> MDYKDDDDKDYKDDDDKDYKDDDDKLEVLFQGPGMSFKATITESGKQNIWFRAIYVLSTIQDDIKITVTTNELIAWSMNETDTTLCQVRFQKSFFEEYEFKPHEIVFGENGVQVIEDTYGNSHKLYSFRVNGRHLTTISRKPDGDGIKSFTIAVNNTSTCPESLANRLIVVIEMDSLIVKEYCPQFQPIKYDPIIINLKYKRRFLDVFGTAASDRNPQEPLDPKLLDVFTNTERELTSALFNEEVESDIRKRNQLTAADEINYICCNSTLLKNFLDNCNVNVTDEVKLEINVHRLSITAFTKAVYGKNNDLLRNALSMSNTISTLDLEHYCLFTTIEDEKQDKRSHSKRREHMKSIIFKLKDFKNFITIGPSWKTTQDGNDNISLWFCHPGDPILMQMQKPGVKLELVEVTDSNINDDILEGKFIKTAISGSKEEAGLKDNKESCESPLKSKTALKRENLPHSV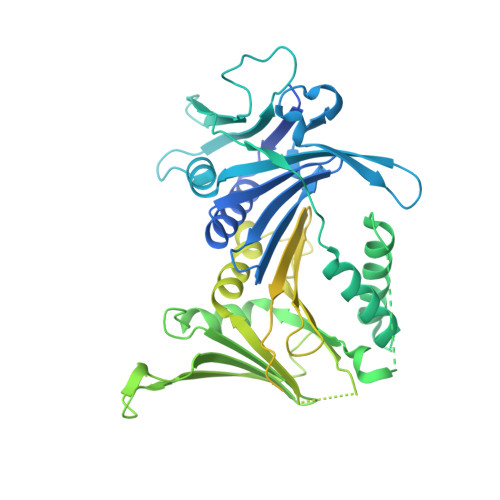AGTRNSPLKVSYLTPDNGSTVAKTYRNNTARKLFVEEQSQSTNYEQDKRFRQASSVHMNMNREQSFDIGTTHEVACPRNESNSLKRSIADICNETEDPTQQSTFAKRADTTVTWGKALPAADDEVSCSNIDRKGMLKKEKLKHMQGLLNSQNDTSNHKKQDNKEMEDGLGLTQVEKPRGIFD> MASVHGTTYELLRRQGIDTVFGNPGSNELPFLKDFPEDFRYILALQEACVVGIADGYAQASRKPAFINLHSAAGTGNAMGALSNAWNSHSPLIVTAGQQTR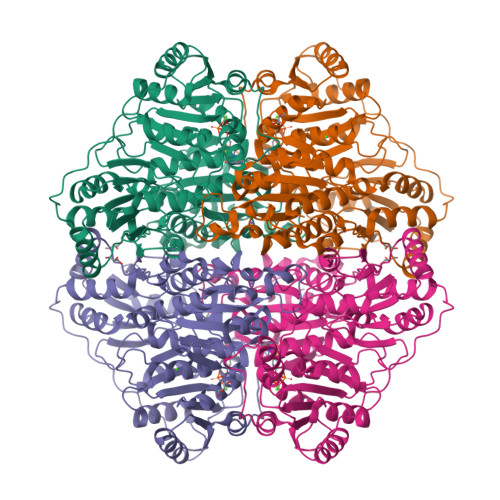AMIGVEALLTNVDAANLPRPLVKWSYEPASAAEVPHAMSRAIHMASMAPQGPVYLSVPYDDWDKDADPQSHHLFDRHVSSSVRLNDQDLDILVKALNSASNPAIVLGPDVDAANANADCVMLAERLKAPVWVAPSAPRCPFPTRHPCFRGLMPAGIAAISQLLEGHDVVLVIGAPVFRYHQYDPGQYLKPGTRLISVTCDPLEAARAPMGDAIVADIGAMASALANLVEESSRQLPTAAPEPAKVDQDAGRLHPETVFDTLNDMAPENAIYLNESTSTTAQMWQRLNMRNPGSYYFCAAGGSGFALPAAIGVQLAEPERQVIAVIGDGSANYSISALWTAAQYNIPTIFVIMNNGTYGALRWFAGVLEAENVPGLDVPGIDFRALAKGYGVQALKADNLEQLKGSLQEALSAKGPVLIEVSTVSPVKRSHHHHHH> 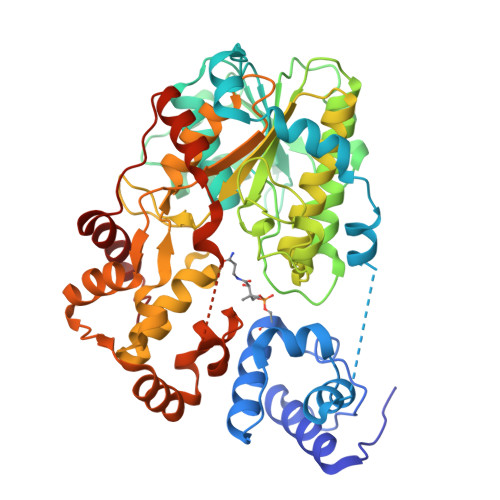GSGAVELNYVAPKTRLEHEICAIFSSILNIETVGVEDNFFEIGGTSLIASKLIIELLKQGYSVRYDDIFRNKTPRALAKLLSGEDIGEEDLDLTDDIIKNYNYGEINELLQENTWENFFDGENLELGNVLLTGATGFLGIHILYEFIKSEEGKIYCMLRKGKFDSCQERLIDVMNDYFDEDFTDLVGSRIIPIEGDITEIDDFKQLEDEPIDTVINSAALVKHYTADDYIFRVNVDGVINGLKFAQTRNNIKYVQISTISVLSSYSLNEEAYPNQEYDERTLYYEQDLENKYVCSKFLAERAVLQAATKGLPVKIIRVGNLMSRYSDGVFQKNYDTNAFLNNIKTIKKLGAMNPAMASEKVDMSQIDYVAKGILALSKTPEKSRVFHCMNNHYISHRDIVDALNTYGYGIEEVDFEEFKQIYEQNMNENIQGIITADFSIDDFDEEDDFEENVEIEQTVDILHSLGFDWPEADEEYLKRLFDYLNKFDYFE RfaH, a paralog of the universally conserved NusG, binds to RNA polymerases (RNAP) and ribosomes to activate expression of virulence genes. In free, autoinhibited RfaH, an α-helical KOW domain sequesters the RNAP-binding site. Upon recruitment to RNAP paused at an ops site, KOW is released and refolds into a β-barrel, which binds the ribosome. RfaH recruitment requires a 12-nucleotide (nt) operon polarity suppressor (ops) sequence, which induces RNAP pausing.

To follow the complete RfaH recruitment and activation, we determined cryoEM/SPA structures of opsPECs assembled on c- and nc-scaffolds with RfaHwt. To facilitate possible conformational changes, we incubated the samples at 37 °C for 10 min before vitrification and imaging.

>[2x]MQGSVTEFLKPRLVDIEQVSSTHAKVTLEPLERGFGHTLGNALRRILLSSMPGCAVTEVEIDGVLHEYSTKEGVQEDILEILLNLKGLAVRVQGKDEVILTLNKSGIGPVTAADITHDGDVEIVKPQHVICHLTDENASISMRIKVQRGRGYVPASTRIHSEEDERPIGRLLVDACYSPVERIAYNVEAARVEQRTDLDKLVIEMETNGTIDPEEAIRRAATILAEQLEAFVDLRDVRQPEVKEEKPEFDPILLRPVDDLELTVRSANCLKAEAIHYIGDLVQRTEVELLKTPNLGKKSLTEIKDVLASRGLSLGMRLENWPPASIADE;> MVYSYTEKKRIRKDFGKRPQVLDVPYLLSIQLDSFQKFIEQDPEGQYGLEAAFRSVFPIQSYSGNSELQYVSYRLGEPVFDVQECQIRGVTYSAPLRVKLRLVIYEREAPEGTVKDIKEQEVYMGEIPLMTDNGTFVINGTERVIVSQLHRSPGVFFDSDKGKTHSSGKVLYNARIIPYRGSWLDFEFDPKDNLFVRIDRRRKLPATIILRALNYTTEQILDLFFEKVIFEIRDNKLQMELVPERLRGETASFDIEANGKVYVEKGRRITARHIRQLEKDDVKLIEVPVEYIAGKVVAKDYIDESTGELICAANMELSLDLLAKLSQSGHKRIETLFTNDLDHGPYISETLRVDPTNDRLSALVEIYRMMRPGEPPTREAAESLFENLFFSEDRYDLSAVGRMKFNRSLLREEIEGSGILSKDDIIDVMKKLIDIRNGKGEVDDIDHLGNRRIRSVGEMAENQFRVGLVRVERAVKERLSLGDLDTLMPQDMINAKPISAAVKEFFGSSQLSQFMDQNNPLSEITHKRRISALGPGGLTRERAGFEVRDVHPTHYGRVCPIETPEGPNIGLINSLSVYAQTNEYGFLETPYRKVTDGVVTDEIHYLSAIEEGNYVIAQANSNLDEEGHFVEDLVTCRSKGESSLFSRDQVDYMDVSTQQVVSVGASLIPFLEHDDANRALMGANMQRQAVPTLRADKPLVGTGMERAVAVDSGVTAVAKRGGVVQYVDASRIVIKVNEDEMYPGEAGIDIYNLTKYTRSNQNTCINQMPCVSLGEPVERGDVLADGPSTDLGELALGQNMRVAFMPWNGYNFEDSILVSERVVQEDRFTTIHIQELACVSRDTKLGPEEITADIPNVGEAALSKLDESGIVYIGAEVTGGDILVGKVTPKGETQLTPEEKLLRAIFGEKASDVKDSSLRVPNGVSGTVIDVQVFTRDGVEKDKRALEIEEMQLKQAKKDLSEELQILEAGLFSRIRAVLVAGGVEAEKLDKLPRDRWLELGLTDEEKQNQLEQLAEQYDELKHEFEKKLEAKRRKITQGDDLAPGVLKIVKVYLAVKRRIQPGDKMAGRHGNKGVISKINPIEDMPYDENGTPVDIVLNPLGVPSRMNIGQILETHLGMAAKGIGDKINAMLKQQQEVAKLREFIQRAYDLGADVRQKVDLSTFSDEEVMRLAENLRKGMPIATPVFDGAKEAEIKELLKLGDLPTSGQIRLYDGRTGEQFERPVTVGYMYMLKLNHLVDDKMHARSTGSYSLVTQQPLGGKAQFGGQRFGEMEVWALEAYGAAYTLQEMLTVKSDDVNGRTKMYKNIVDGNHQMEPGMPESFNVLLKEIRSLGINIELEDE;> VKDLLKFLKAQTKTEEFDAIKIALASPDMIRSWSFGEVKKPETINYRTFKPERDGLFCARIFGPVKDYECLCGKYKRLKHRGVICEKCGVEVTQTKVRRERMGHIELASPTAHIWFLKSLPSRIGLLLDMPLRDIERVLYFESYVVIEGGMTNLERQQILTEEQYLDALEEFGDEFDAKMGAEAIQALLKSMDLEQECEQLREELNETNSETKRKKLTKRIKLLEAFVQSGNKPEWMILTVLPVLPPDLRPLVPLDGGRFATSDLNDLYRRVINRNNRLKRLLDLAAPDIIVRNEKRMLQEAVDALLDNGRRGRAITGSNKRPLKSLADMIKGKQGRFRQNLLGKRVDYSGRSVITVGPYLRLHQCGLPKKMALELFKPFIYGKLELRGLATTIKAAKKMVEREEAVVWDILDEVIREHPVLLNRAPTLHRLGIQAFEPVLIEGKAIQLHPLVCAAYNADFDGDQMAVHVPLTLEAQLEARALMMSTNNILSPANGEPIIVPSQDVVLGLYYMTRDCVNAKGEGMVLTGPKEAERLYRSGLASLHARVKVRITEYEKDANGELVAKTSLKDTTVGRAILWMIVPKGLPYSIVNQALGKKAISKMLNTCYRILGLKPTVIFADQIMYTGFAYAARSGASVGIDDMVIPEKKHEIISEAEAEVAEIQEQFQSGLVTAGERYNKVIDIWAAANDRVSKAMMDNLQTETVINRDGQEEKQVSFNSIYMMADSGARGSAAQIRQLAGMRGLMAKPDGSIIETPITANFREGLNVLQYFISTHGARKGLADTALKTANSGYLTRRLVDVAQDLVVTEDDCGTHEGIMMTPVIEGGDVKEPLRDRVLGRVTAEDVLKPGTADILVPRNTLLHEQWCDLLEENSVDAVKVRSVVSCDTDFGVCAHCYGRDLARGHIINKGEAIGVIAAQSIGEPGTQLTMRTFHIGGAASRAAAESSIQVKNKGSIKLSNVKSVVNSSGKLVITSRNTELKLIDEFGRTKESYKVPYGAVLAKGDGEQVAGGETVANWDPHTMPVITEVSGFVRFTDMIDGQTITRQTDELTGLSSLVVLDSAERTAGGKDLRPALKIVDAQGNDVLIPGTDMPAQYFLPGKAIVQLEDGVQISSGDTLARIPQESGGTKDITGGLPRVADLFEARRPKEPAILAEISGIVSFGKETKGKRRLVITPVDGSDPYEEMIPKWRQLNVFEGERVERGDVISDGPEAPHDILRLRGVHAVTRYIVNEVQDVYRLQGVKINDKHIEVIVRQMLRKATIVNAGSSDFLEGEQVEYSRVKIANRELEANGKVGATYSRDLLGITKASLATESFISAASFQETTRVLTEAAVAGKRDELRGLKENVIVGRLIPAGTGYAYHQDRMRRRAAGEAPAAPQVTAEDASASLAELLNAGLGGSDNELEVHHHHHH;> MARVTVQDAVEKIGNRFDLVLVAARRARQMQVGGKDPLVPEENDKTTVIALREIEEGLINNQILDVRERQEQQEQEAAELQAVTAIAEGRR;> GHMQSWYLLYCKRGQLQRAQEHLERQAVNCLAPMITLEKIVRGKRTAVSEPLFPNYLFVEFDPEVIHTTTINATRGVSHFVRFGASPAIVPSAVIHQLSVYKPKDIVDPATPYPGDKVIITEGAFEGFQAIFTEPDGEARSMLLLNLINKEIKHSVKNTEFRKL>MNHKVHHHHHHIEGRHMKVNISIFGFGTVGRALAEIIAEKSRIFGVELNVISITDRSGTIWGDFDLLEAKEVKESTGKLSNIGDYEVYNFSPQELVEEVKPNILVDVSSWDEAHEMYKVALGEGISVVTSNKPPIANYYDELMNLAKENNAGIFFESTVMAGTPIIGVLRENLLGENIKRIDAVVNASTTFILTKMSEGKTLDDAIEEAKSLGILEEDPSKDIDGIDAYYKAKILHWVSYGEPPEEEERLGIREVRDARNVRLVAQVSKGKISVKPRKLSSDNPLLVEGVQNAAVIRTNNLGEVILKGPG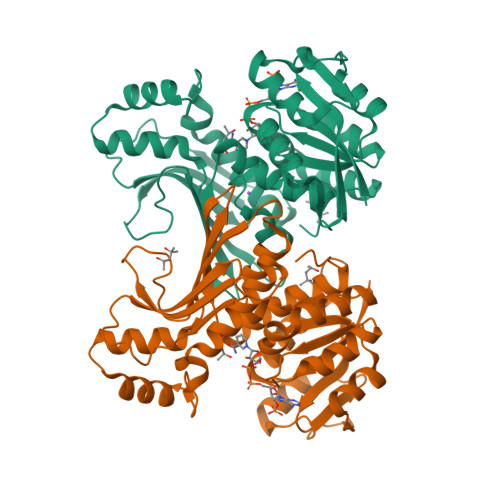GGGRVTASGVFTDIIKATLKFPNLR[2x]4-(difluoromethyl)-5-{4-[(3S)-3-methylmorpholin-4-yl]-6-(morpholin-4-yl)-1,3,5-triazin-2-yl}pyridin-2-amine 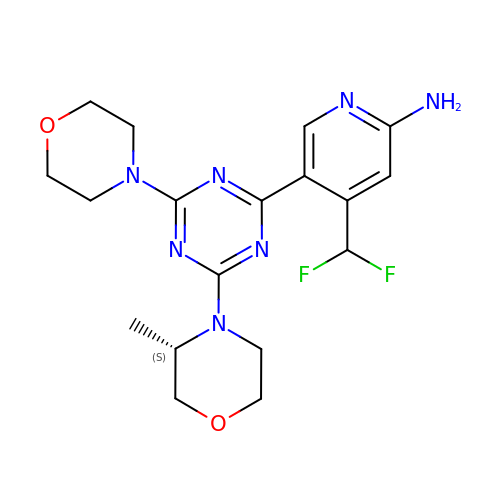| C18 H23 F2 N7 O2 | SYKBZXMKAPICSO-NSHDSACASA-N> MHLKIVCLSDEVREMYKNHKTHHEGDSGLDLFIVKDEVLKPKSTTFVKLGIKAIA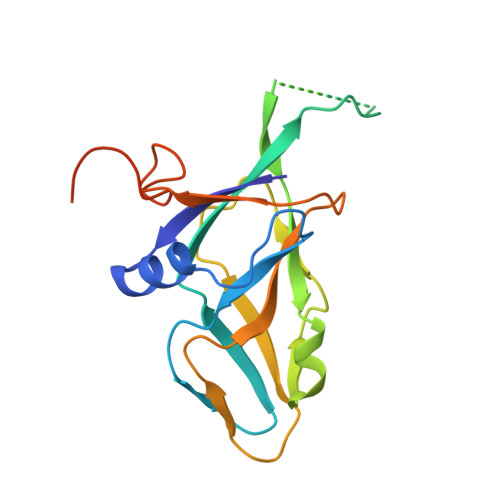LQYKSNYYYKCEKSENKKKDDDKSNIVNTSFLLFPRSSISKTPLRLANSIGLIDAGYRGEIIAALDNTSDQEYHIKKNDKLVQLVSFTGEPLSFELVEELDETSRGEGGFGSTSNNKYEAHHHHHH>[2x]MEVHAADQYLVAPGEADLLEVHARLAGTGLFPPFPPVELPGGVGGLVARGGFAQTFFFPAEVLGLTFRTPKGRRVRAGG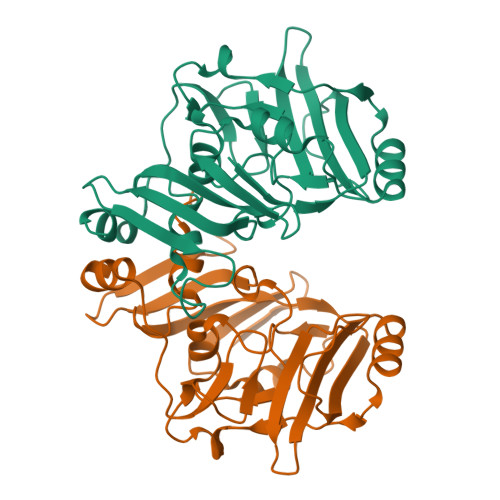VVVKNVQGYDLVRLFVGSFGLLGRAEEVVLRLRPGRAQAFLRRPFSGSFPRLVPTPRFLFALEDEEGPWLYAYHFGHPKEVERFREAFGGEEARPLDLRPRFPRGLGLGEGPLWDLRFRYQDGGASPPPPPAFLRLARVL> PA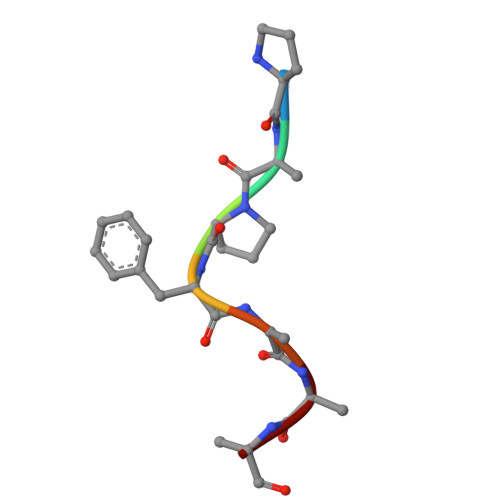PFAAA>[4x]GSMGRIADSRLLWDYVYQLLSD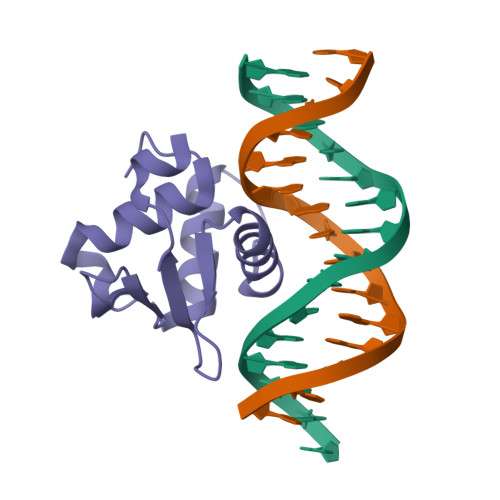SRYENFIRWEDKESKIFRIVDPNGLARLWGNHKNRTNMTYEKMSRALRYYYKLNIIRKEPGQRLLFRFMKTPDEIMSGR>[2x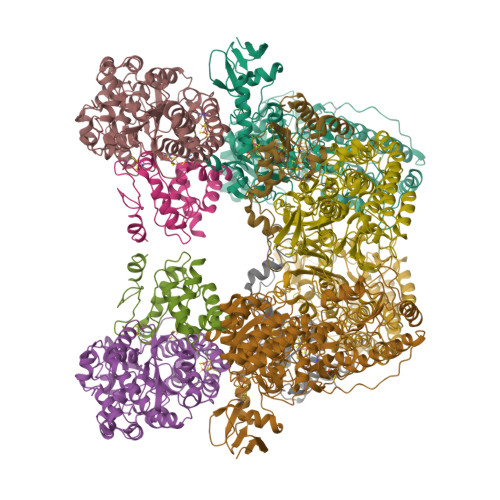]MKEITLTIDGKVCKGVQGDTILDVANKNDVYIPTLCYQKGLTPIGACRMCVVQLEGNPKMLPSCTTPAQDGMVVVTKNEKLKDYRRQILELLFAGRNHFCMYCSQSGDCELQRLAIEHEMDSVRFPYLYEDFEVDATDPNLMMDHNRCVLCQRCIRTCSEIVGAHTLDLERRGWQAKVIADLGKRLRESDTCVNCGACAQSCPTGTITIREFAYRGRRSECDAVVESVCPLCAVGCKIKTYVRTGSIVRVEGTGVEEPDGGQLCHMGRWWLPESTERERVTVPLIREGASYREATWEEALALASAEFKKAYDQEKAGAILSSLCTDEELTLFSALFRNALKMKHIDTFDGDIIRGFFKGFMPFREQGVRPFTAAHHILDSDLIITMFADPQKEAPVVASYIRVACLHRNAKLMNLSYGPSPFPGLVDLDIRLPEGQAVPKALSNLAEIIGKISLGPSDMASFGEFEAGAGKALSSYRESIEESARAMGLDPKIAEEVALMLISARRPIFIIGGRATKSHELVTAACNLAVASKAFFEDGLGVVPLLVSANSLGARNTVVSENPWLGRERRDFLYVFSTAMVPEEEEILAAISATRFVVVQTPFKVRPLVNLADILLPAPAWYERSGHFCTIEGERRKLNTIVPPKGEIKSLHYVMDEFAKKLGVKLERPEVSPCEEIFKSQLRASEARIVTL;>MAIYRAHVLVCRGTGCTASGAPGVMKAFKEELAKKGLDREVMLVETGCHGMCEMGPVVVVYPEGAFYCRVTPEDVPEIVEEHLYKGRIVQRLLYTVPEDMEKVPYYKDIPFYSKQHRIVLSNCGYIDPEKIEEYIARDGYMALGKALLEMTPEEVLEEVKKSGLRGRGGAGFPTGLKWEFAKKASGDKKYVICNADEGDPGAFMDRSTLEGDPHSVIEGMTIGAYVIGADEGYIYCRAEYPLAIKRLKIAIAQAEEMGLLGDHIMGTNFSFHLHLKEGAGAFVCGEETALMASIEGRRGMPRPRPPFPAQHGLWGKPTNINNVETWANVPRIILNGADWFASMGTEKSKGTKIFALTGKITNTGLIEVPMGITIREIIYELGGGILNGKEFKAVQIGGPSGGCLTKEHLDLPIDYESLTAAGAIMGSGGLVVMDEDTCMVDVAKFFLEFTQRESCGKCVPCREGTKQMLLMLQKICNGEGTMDDLSKLEELAHMVKETSLCGLGQTAPNPVITTIRYFRDEYVAHIKDKRCPAKICPALIKYVVDPEKCRKCGLCARNCPVKCISGDRQTPYLINQEKCIKCGTCMQVCPFGAIGKV[2x];>MALSTVDVVEKVKEIVAPWKGKQGGLIPILQEVQRELGYLPEEALLTISRELKMPKAEVYGVATFYAQFHLKPRGRHVIRVCRGTACHVRGSLQILEKVKQMLGIEENETTDDLRFTLEPVACLGACGLAPVMMVDEDTHGRMTPDKIQAILDKYQ[2x];>[2x]MTEVFKLEINPVTRIEGHGKITVMLDESGHVRETRFHVTQYRGFEVFTHGRDFREMPVITPRICGICPVSHHLASAKACDEILGVTITPAAHKLRELMHMGQIVQSHALSFFHLSSPDILWGFDAPVKIRNVAGLVDRYPELAKKGIMLRKFGQEIIKTLGGKKIHPWHSIPGGVNRSLTPQERDAIAAQLPEMKSIAMEAIKLIKDYLQEGGEELKEFATLDTAYMGLVRDGYLELYDGEVRIKAPRGRILDQFDPKDYLDHIGEHVEPWSYLKFPFYKALGFPHGSYRVGPLARLNAADAVSTPEASKEFALYKEMGEDGIVPYTLYYHYARLIEALYGLERIEQLLADPDITSSDLRVTSKEINPEGIGVIEAPRGTLIHHYQVNESGVITKVNLIVATGHNNFAMNKGVEMVAKKYITGTNVPEGVFNRLEHVIRAYDPCLSCSTHAVGKMPLKLELVGPTGEILKEVTRD;>[2x]MAKAKVATFWLEACAGCHMSFLDLDERLIDLFQNVEILFSPIVDAKDIPNIDVGVLSGGLGNVEEVELAKKMRERCKYLVAWGDCAVFGGINCMRNFIPKDVVLREGYIETASTVNPQGIVPSEDIPELLPRALPIDYEVKVDVYVPGCPPDADTIYYVFKELLAGRVPKVPSEMMRYD RFCCtf18 is a seven‐subunit complex formed of Ctf18, Rfc2‐5 and the stable Dcc1‐Ctf8 sub‐complex. The complex is required for activation of the intra‐S‐phase checkpoint and proper establishment of sister chromatid cohesion. RFCCtf18 is a variant replication factor C‐like complex, the basic function of which is to load or unload a DNA sliding clamp in an ATP‐dependent manner 19, 20. Previous studies have shown that Dcc1 and Ctf8 are able to form a stable sub‐complex in vitro and that the C‐terminus of Ctf18 is required for the interaction with the Dcc1‐Ctf8 sub‐complex 39.

While working on this complex, we also obtained crystals of the C‐terminal domain of Dcc1 (residues 90–380) that diffracted to 2 Å. Phase information for this crystal form was determined using multiple‐wavelength anomalous diffraction (MAD) of selenomethionine‐substituted protein. The refined structure was then used as a search model to determine the structure of the Ctf18C‐Dcc1‐Ctf8 heterotrimer by molecular replacement (MR). To identify whether any common domains were present in the heterotrimer, we performed a three‐dimensional homology search using the Dali server 48. The results indicated that Dcc1 contains three‐winged helix (WH) domains from residues 182–252, 253–317 and 318–380, which we have called WH1, WH2 and WH3, respectively. A large conserved basic patch was present on the surface of WH3. This suggested the domain could interact with DNA as basic residues are able to bind to the negatively charged backbone of DNA. A gel shift was observed with both ssDNA and dsDNA, suggesting Dcc1 could interact with both substrates. Mutation of K364, R367 or R380 reduced the affinity for both ssDNA and dsDNA, albeit weakly with K364, while the triple mutant K364A, R367A, R380A totally eliminated binding similar to the WH3 deletion. These residues are widely conserved and suggest that the binding site for ssDNA and dsDNA overlaps to some extent.

>[4x]GSGLSKPYMDVVGFAKTESEFETRETHGELNLNSVPIYNGELDFSDKIMKRSSTKVIGTLEELLENSPCSALEGISKWHKIGGSVKDGVLCILSQDFLFKALHVLLMSAMAESLDLQHLNVEDTHHAVGKDIEDEFNPYTREIIETVLNKFAVQEQEAENNTWRLRIPFIAQWYGIQALRKYVSGISMPIDEFLIKWKSLFPPFFPCDIDIDMLRGYHFKPTDKTVQYIAKSTLPMDPKERFKVLFRLQSQWDLEDIKPLIEELNSRGMKIDSFIMKYARRKRLGKKTVVTSR> MISNEEQTPLLKKINPTESTSKAEENEKVDSKVKAFKKPLSVFKGPLLHISPAEELYFGSTESGE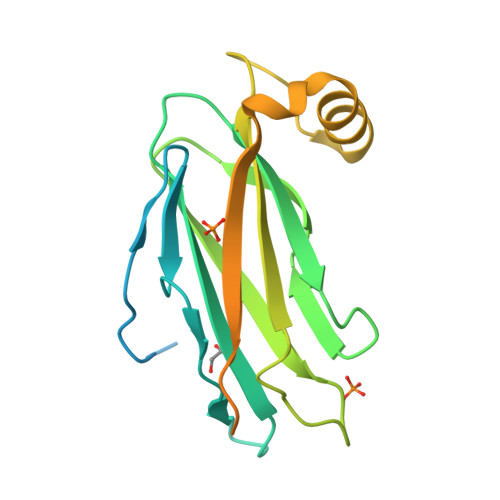KKTLIVLTNVTKNIVAFKVRTTAPEKYRVKPSNSSCDPGASVDIVVSPHGGLTVSAQDRFLIMAAEMEQSSGTGPAELTQFWKEVPRNKVMEHRLRCHTVESSKPNTLTLKDNAFNMSDKTSEDICLQLSRLLESNRKLEDQVQRHHHHHH> MGSYLHEPPGDEPSMRIEQPKTADRAPEQVAIHICEPSKVVTESFPFSETAEPEAKSKNCPCPEIARIGPCPNKPPKIPINRGLSRISTNKSRPKSRFGEPSWPVESSLDLTSQSPVSPYREEAFSVENCGTAGSRRGSFARGTTSRAASSSRKDETKEGPDEKEVYQRVTAQLSARNQKRMTVKLMIELSVFLCLLGCLVCSLTVDGFKRYTVIGLDIWKWFLLLLVIFSGMLITHWIVHVAVFFVEWKFLMRKNVLYFTHGLKTSVEVFIWITVVLATWVMLIKPDVNQPHQTRKILEFVTWTIVTVLIGAFLWLVKTTLLKILASSFHLNRFFDRIQESVFHHSVLQTLAGRPVVELAQGISRTESQDGAGQVSFMEHTKTQNKKVVDVGKLHQMKQEKVPAWTMQLLVDVVSNSGLSTMSGMLDEDMVEGGVELDDDEITNEEQAIATAVRIFDNIVQDKVDQSYIDRVDLHRFLIWEEVDHLFPLFEVNEKGQISLKAFAKWVVKVYNDQAALKHALNDNKTAVKQLNKLVTAILIVMMIVIWLIVTGIATTKLIVLLSSQLVVAAFIFGNTCKTIFEAIIFVFVMHPFDVGDRCVIDGNKMLVEEMNILTTVFLKWDKEKVYYPNSILCTKAIGNFFRSPDQGDVLEFSVDFTTPVLKIGDLKDRIKMYLEQNLNFWHPQHNMVVKEIENVNKIKMALFVNHTINFQDFAEKNRRRSELVLELKKIFEELDIKYNLLPQEISIRNMGSGSLEVLFQ

Flycatcher1 (FLYC1), a MscS homolog, has recently been identified as a candidate mechanosensitive (MS) ion channel involved in Venus flytrap prey recognition. FLYC1 is an ortholog of prokaryotic MS ion channel MscS (mechanosensitive ion channel of small conductance), which functions as an osmotic release valve, and is perhaps the most extensively studied MS channel. FLYC1 comprises a homoheptamer with six TMs (TM1–TM6) per protomer and intracellular N and C termini. A glycine-containing hinge (G575) splits TM6 into two halves (TM6a and TM6b), and the β-rich C-termini of the FLYC1 protomers come together to form a hollow cytoplasmic cage.

C7 symmetry expansion followed by focused classification and refinement of the peripheral region yielded two distinct classes with improved density. The two classes are referred to as either ‘up’ or ‘down’ based on the orientation of two cytoplasmic helices that extend from the transmembrane domain (TMD). In our dataset, protomers favored the up over the down class, with approximately 72 and 16% of the symmetry expanded particles assigned to each class, respectively. The molecular model of FLYC1 was initially built from the best-resolved of the two classes, the up class, which was the primary subject of our structural analysis unless otherwise stated. In the up conformation, the TM4-TM5 linker is parallel to the membrane plane, while in the down conformation, the linker swivels towards the cytosol. In the up state, the cytosolic extension of TM4 interacts with the β-domain of the cytoplasmic cage through a salt bridge between R334 and D598 (2.9 Å distance). To test this, we disrupted the R334–D598 salt bridge by either mutating the arginine to glutamate or mutating the aspartate to lysine and determined its effect on channel kinetics. D598K mutation rendered the channel non-functional, but remarkably, stretch-activated currents from R334E mutant exhibited a drastic increase in open-dwell time in both macroscopic and single-channel currents. Effectively, the deactivation time constant of the channel was approximately 40-fold slower than WT (WT: 0.477 ± 0.285 s (N = 6); R334E: 18.5 ± 5.2 s (N = 6)). The striking 40-fold delay in deactivation kinetics upon disruption of the up state-specific R334–D598 interaction suggests that the formation of this salt bridge in the WT protein is associated with channel closure and that losing this interaction is important for the stability of the open state.>[2x]DTHTPEFLGDSSNSGLWPNGNYGEDIIIGVLDTGVWPEHPSFSDSDMSDIPSSWKGTCETSDDFPASSCNKKLIGARAFSKGIVAYQGAPIDKSKDSDSPRDINGHGTHTSTTAGGSKVQNASFYGYAKGQARGMATKARIAVYKVCWSAGCPDTDILAAMNQAIEDGVHVISMSVGPQGYSPDYYQEASAIGAFNAVKYGIIVSCSAGNSGPKPLTAGNISPWILTVGASTIDREFRADVVLGDGRTFKG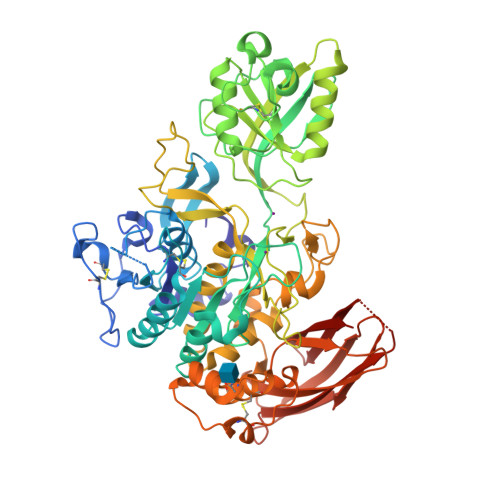SSLYTGEPLQDEFFPLVYAGYAGSSRFCTNGSLDSSKVQGKIVICDNGIISREEKGNEVNRAGGAGMIDVTAEDFLRAGDAYLFPATTVTLTDGYEIEYYSVTSQSPTAKIVFLGTVIGNSPPAPKVASFSSRGPNLWTPQILKPDVIAPGVAILAGWSGAAHPTDLDNDDRIVQFWLDSGTSMACPHVSGIVALLRKAHPSWSAAAIKSALMTTAYNLDNSGETITDVATSNASTPFDRGAGHVHPDSALDPGLVYDSDTEDYVSFLCAIGYNSTLIGIFTGEVPPSDICDNYKLGSPGNLNYPSFSVAFEGDTSNVTYKRTVTNVGSSSDVVYRVKVNAPPSVDVSVSPSSLVFSKENPSLSYEITFTSTLXXXXXXAQSFGSIEWSDGTHSVRSPIAIDW>[2x]MQGVNIYNISAGTSVDLAAPVTTGDIVTFFSSAANLNAGAGNPNNTTLNLFAENGAYLLHIAFRLQENVIIF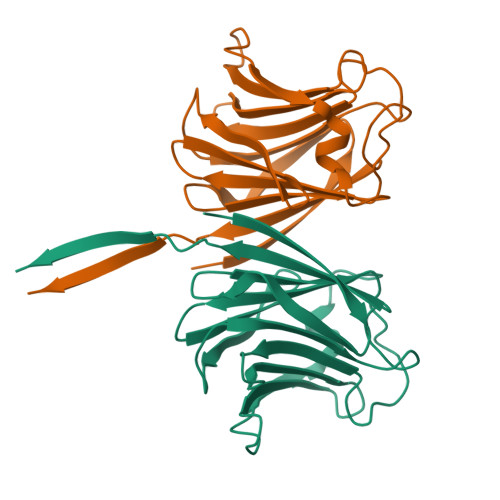NSRQPDGPWLVEQRVSDVANQFAGIDGKAMVTVFDHGDKYQVVINEKTVIQYTKQISGLTSSLSYNATEETSIFSTVVEAVTYTGLALEHHHHHH> GGAUCGCUAGGGUUCCGGUCGUGCGGCGUUCGCGCCGCACGAUGCUGGUCCGAGAGCAAUCCGGUCUUGCCUUCGCCUCGUUCGCGAGGAAACGGCGAGGCUCCACGGAGGGAUAAAAGCCCGGG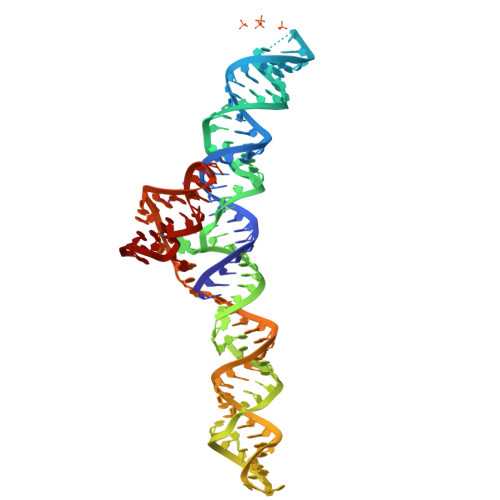AGG heptyl 2-deoxy-alpha-D-mannopyranoside 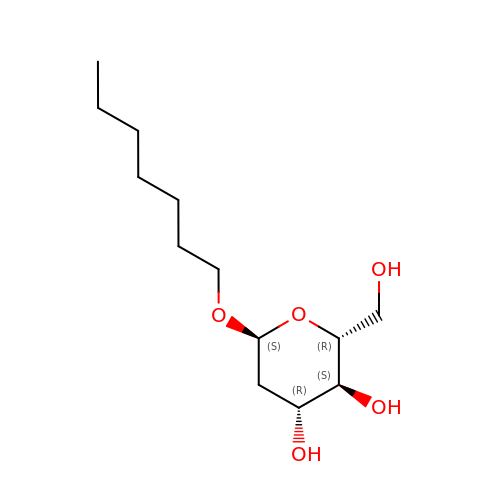| C13 H26 O5 | IRECALVMQPMJAW-NDBYEHHHSA-N> MYGDLGNKLVLEAKRTKQLYARSNQDVNLPMYHEDIIRNILKEVSNLRKNTEYLKEQQQLGMLDDKVAKCQYFVTLLCMERNKRCLLA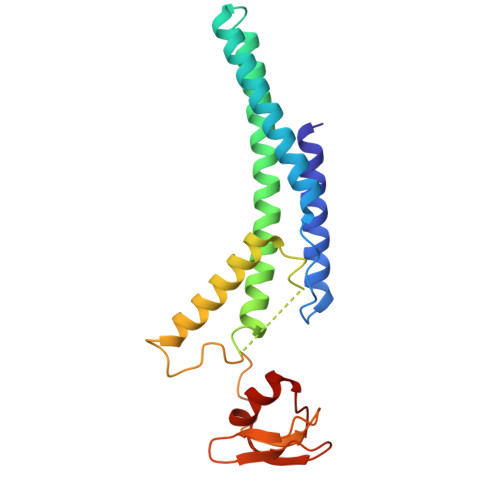YQRLRTDILDSMAWNNNGLDLMSSITFSQQDTNNLSHQEQEYLKEYCDLITDLKSGDLVDIDLSGSLVPPSDVFIDVRVLKDAGEIQTEYGVFNLIKDSQFFVRQSDVERLIQQGYLQKI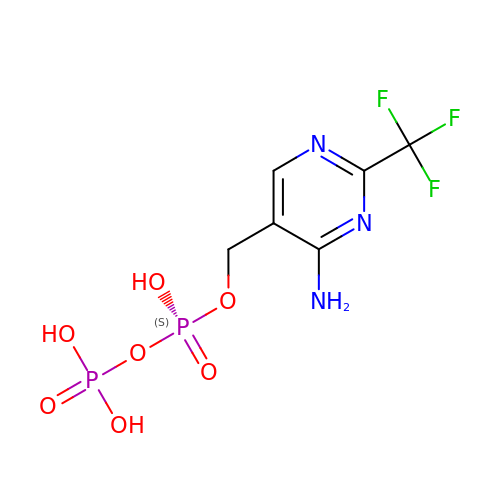4-AMINO-2-TRIFLUOROMETHYL-5-HYDROXYMETHYLPYRIMIDINE PYROPHOSPHATE | C6 H8 F3 N3 O7 P2 | UKNJCTHTCAKKNG-UHFFFAOYSA-N> MRSYPAIPRIYAETTLNMLLKRAKKPRVHSIDEYLKDGGYQALEKALNMSPEEIIDWVDKSTLRGRGGAGFPTGKKWKFAVQNPGPRYFICNADEMEPGTFKDRIIIERDPHLLIEGIIISSYAIGANEAYIYIRGEYPAGYYILRDAIEEAKKKGFLGKNILGSGFDLEIYVARGAGAYICGEETALI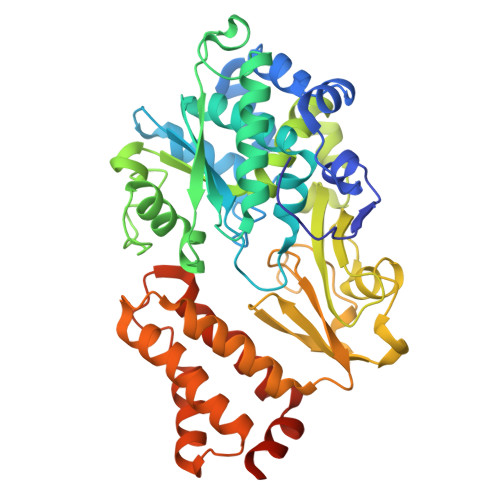ESLEGKRGHPRLKPPYPVQKGLWGKPTVVNNVETIANVPFIISMGWEEYRYIGPSDYAGPKLFPVSGKVKKPGVYELPMNTTLREVIFKYAGGTLGNKKVKAVFSGALDCFSSEELDIPMDYSPLGFGGTGTVIVLTEEDDIVEAALKIAEFYEHETCGQCTPCRVGCYEQANLLEKIYKGEATEQDWEGFDFVNRNIQPTSICGLGAVAGRLIRQTLEKFPEEWEKYRKKSASLPLAGHHHHHH benzyl 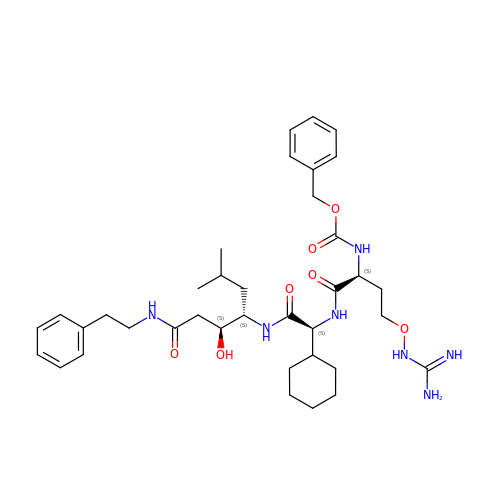[(6S,7S,10S,13S,18Z)-18-amino-10-cyclohexyl-6-hydroxy-18-imino-7-(2-methylpropyl)-4,9,12-trioxo-1-phenyl-16-oxa-3,8,11,17-tetraazaoctadecan-13-yl]carbamate | C37 H55 N7 O7 | QUXHBSKCTRDCOH-QUUJSONZSA-N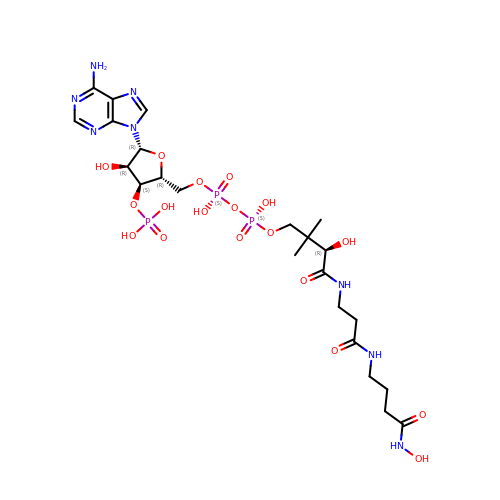N-HYDROXYAMIDOCARBOXYMETHYLDETHIA COENZYME *A | C23 H39 N8 O18 P3 | UCBQLSAQGRRAIX-GRFIIANRSA-N> MKTTSFILALIISISIGKAQTNHQVSYFSLQDVKLLSSPFLQAQQTDLHYILALDPDRLSAPFLREAGLTPKAPSYTNWENTGLDGHIGGHYLSALSMMYAATGDTAIYHRLNYMLNELHRAQQAVGTGFIGGTPGSLQLWKEIKAGDIRAGGFSLNGKWVPLYNIHKTYAGLRDAYLYAHSDLARQMLIDLTDWMIDITSGLSDNQMQDMLRSEHGGLNETFADVAEITGDKKYLKLARRFSHKVILDPLIKNEDRLNGMHANTQIPKVIGYKRVAEVSKNDKDWNHAAEWDHAARFFWNTVVNHRSVCIGGNSVREHFHPSDNFTSMLNDVQGPETCNTYNMLRLTKMLYQNSGDVDNSNKPDPRYVDYYERALYNHILSSQEPDKGGFV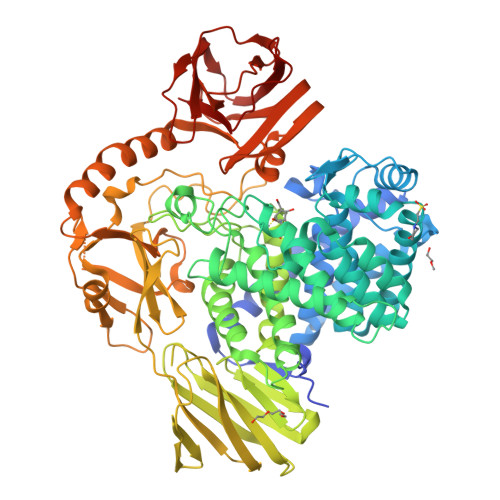YFTPMRPGHYRVYSQPETSMWCCVGSGLENHTKYGEFIYAHQQDTLYVNLFIPSQLNWKEQGVTLTQETLFPDDEKVTLRIDKAAKKNLTLMIRIPEWAGNSKGYEITINGKKHLSDIQTGASTYLPIRRKWKKGDMITFHLPMKVSLEQIPDKKDYYAFLYGPIVLATSTGTENLDGIYADDSRGGHIAHGRQTPLQEIPMLIGNPDSIRHSLHKLSGSKLAFSYDGNVYPTQKSKSLELIPFFRLHNSRYAVYFRQASEEQFKTIQEEMATAERKATELANRTVDLIFPGEQQPESDHSIQYEASETGTHKDRHFRRAKGWFSYNLKIKEEASQLMITVRQEDRNKAVILLNNEKLTVHPTVSKADKDGFIRLCYLLPRKLKVGSCEILFKPDGTEWTSAVYEVRLLK> MHHHHHHSSRENLY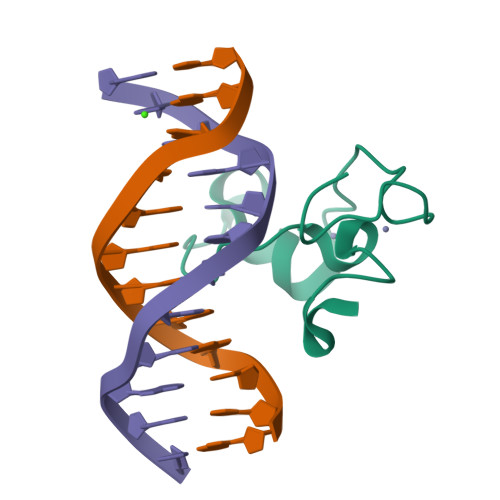FQGQIKRSARMCGECEACRRTEDCGHCDFCRDMKKFGGPNKIRQKCRLRQCQLRARESYKYFPSS> GAMADTTEATPAAAPVAARGGELTQSTHLTLEAATKAARAAVEAAEKDGRHVSVAVVDRNGNTLVTLRGDGAGPQSYDSADRKAFTAVSWNAPTSELAKRLAQAPTLKDIPGTLFLAGGTPVTAKGAPVAGIGVAGAPSGDLDEQYARAGAAVLGH

Our previous reported works have characterized HbpS as the accessory and sensory component of the two-component system SenS-SenR that together mediate a genetic response of Streptomyces against iron- and haem-based oxidative stress. Moreover, studies have shown that HbpS is a novel type of haem-binding protein that degrades haem in vitro and in vivo. In this work, we have shown that this multifunctional extracellular octameric protein binds ferrous iron through D/EXXE signatures. With this sequestration function HbpS complexes ferrous iron from the surrounding environment and oxidizes it to its ferric from, making them inaccessible to react with hydrogen peroxide via the Fenton reaction, the products of which are highly reactive and are damaging to a number of different macromolecules.

To address this point and taking into account that the E78XXE81 motif shows the strongest iron binding, E78D, E81D as well as E78D/E81D mutants were generated. One could expect that the exchange of E to D would not have any significance relevance for iron- binding behaviour, but analyses of isolated mutant proteins incubated with ferrous iron revealed that all three mutants show strong decreased iron-binding activity, namely E78D up to 40.7%, E81D 32% and E78D/E81D 34.9%. In order to gain structural insight into the effects of the E78D and E81D mutations on the iron binding of HbpS, the HbpS-D78XXD81 mutant protein was purified and crystallized. In the wild-type protein, the glutamates (Glu-78 and Glu-81) point towards the central cavity of the octamer and are apposed by the corresponding residues from a second monomer, thus creating a cluster of four negatively charged residues. In the wild-type protein, the distance between the Glu-81 residues from two apposing subunits is 6.7 Å, whereas the distance of the corresponding aspartate residues in the mutant protein is 8.6 Å. Furthermore, in the mutant protein, Asp-81 is engaged in a hydrogen bond with Thr-63, which can be expected to further decrease the ability of this side chain to take part in metal coordination. Moreover, comparative analyses using the high resolution (1.99 Å) crystal structure of HbpS-E78D/E81D and of the wild-type HbpS revealed that the proper orientation and proximity of the side chains of the glutamates from neighbouring E78XXE81 motifs within the octamer are also essential for iron binding. In HbpS-E78D/E81D, the side chains of the aspartates are shortened by one CH2 group, and it can be assumed that this weakens the coordination of an iron. In fact, the iron-binding activity of this mutant is considerably weaker than that from the wild-type. The overall octameric assembly of HbpS-D78XXD81 remains unchanged and no major structural rearrangements were detected.> MGTVSSRRSWWPLPLLLLLLLLLGPAGARAQEDEDGDYEELVLALRSEEDGLAEAPEHGTTATFHRCAKDPWRLPGTYVVVLKEETHLSQSERTARRLQAQAARRGYLTKILHVFHGLLPGFLVKMSGDLLELALKLPHVDYIEEDSSVFAQSIPWNLERITPPRYSADEYQPPDGGSLVEVYLLDTSIQSDHREIEGRVMVTDFENVPEEDGTRFHRQASKCDSHGTHLAGVVSGRDAGVAKGASMRSLRVLNCQGKGTVSGTLIGLEFIRKSQLVQPVGPLVVLLPLAGGYSRVLNAACQRLARAGVVLVTAAGNFRDDACLYSPASAPEVITVGATNAQDQPVTLGTLGTNFGRCVDLFAPGEDIIGASSDCSTCFVSQSGTSQAAAHVAGIAAMMLSAEPELTLAELRQRLIHFSAKDVINEAWFPEDQRVLTPNLV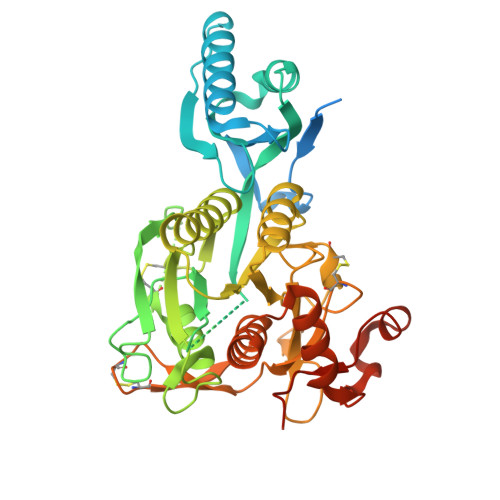AALPPSTHGAGNSHHHHHH Gastric infection by H. pylori depends on the expression of a nickel-dependent urease in the cytoplasm of the bacteria. The ure gene cluster is comprises seven genes, two of which code for a nickel-dependent urease (ureA and ureB) that hydrolyzes urea into NH3 and CO2, one for a pH-gated urea channel (ureI) that delivers host gastric urea to urease in the bacterial cytoplasm, and four for cytoplasmic accessory proteins involved in nickel processing. Ureases (EC 3.5.1.5) are amidohydrolases found in bacteria, algae, plants and fungi with an active site composed of a carbamylated lysine (KCX)14 coordinating a bi-nickel center. The overall single-particle cryo-EM structures of H. pylori urease reveal a 1.1 MDa dodecameric complex of 12 UreA and 12 UreB subunits in a tetrahedral arrangement, in agreement with the previously published crystal structures.

The map at 2.5 Å resolution depicts urease with BME bound in the active site (U-BME) whereas the map at 2.0 Å details the binding of an inhibitor 2-{[1-(3,5-dimethylphenyl)-1H-imidazol-2-yl]sulfanyl}-N-hydroxyacetamide (U-SHA). Briefly, we used the program Relion to obtain maps of U-BME with a resolution of 2.55 Å and of U-SHA with a resolution of 2.09 Å. We determined urease IC50 values under identical conditions for BME and SHA as 13.5 mM and 19.6 μM, respectively. BME coordinates to the two Ni2+ ions through its sulfur in a fashion similar as described for BME binding to Bacillus pasteurii urease, however, we see density for only one BME molecule, whereas Bacillus pasteurii urease shows density for two BME molecules. Nevertheless, BME and the hydroxamic acid moiety of SHA assume similar conformations, probably driven by the requirements of Ni2+ coordination. The structures of H. pylori urease with bound BME and SHA display the same overall fold, with low backbone variations for subunit UreA (below 1 Å), although the C-terminal residues A228-238 show slightly higher root mean square deviation (RMSD) values (below 1.5 Å). The difference in flap region positioning appears to be due to the bulky SHA imidazole and phenyl rings that would sterically clash with the side chains of Cys321 and His322 at the tip of the flap in the BME complex, with both residues fully conserved for the 260 GenBank deposited H. pylori urease sequences.

>MKLTPKELDKLMLHYAGELARKRKEKGIKLNYVEAVALISAHIMEEARAGKKTAAELMQEGRTLLKPDDVMDGVASMIHEVGIEAMFPDGTKLVTVHTPIEANGKLVPGELFLKNEDITINEGKKAVSVKVKNVGDRPVQIGSHFHFFEVNRCLDFDREKTFGKRLDIASGTAVRFEPGEEKSVELIDIGGNRRIFGFNALVDRQADNESKKIALHRAKERGFHGTKSDDNYVKTIKE[12x];>MKKISRKEYVSMYGPTTGDKVRLGDTDLIAEVEHDYTIYGEELKFGGGKTLREGMSQSNNPSKEELDLIITNALIVDYTGIYKADIGIKDGKIAGIGKGGNKDMQDGVKNNLSVGPATEALAGEGLIVTAGGIDTHIHFISPQQIPTAFASGVTTMIGGGTGPADGTNATTITPGRRNLKWMLRAAEEYSMNLGFLAKGNTSNDASLADQIEAGAIGFKIHEDWGTTPSAINHALDVADKYDVQVAIHTDTLNEAGCVEDTMAAIAGRTMHTFHTEGAGGGHAPDIIKVAGEHNILPASTNPTIPFTVNTEAEHMDMLMVCHHLDKSIKEDVQFADSRIRPQTIAAEDTLHDMGIFSITSSDSQAMGRVGEVITRTWQTADKNKKEFGRLKEEKGDNDNFRIKRYLSKYTINPAIAHGISEYVGSVEVGKVADLVLWSPAFFGVKPNMIIKGGFIALSQMGDANASIPTPQPVYYREMFAHHGKAKYDANITFVSQAAYDKGIKEELGLERQVLPVKNCRNITKKDMQFNDTTAHIEVNPETYHVFVDGKEVTSKPANKVSLAQLFSIF[12x]2,4-DICHLORO-6-(3,4,5-TRICHLORO-1H-PYRROL-2YL)PHENOL | C10 H4 Cl5 N O | 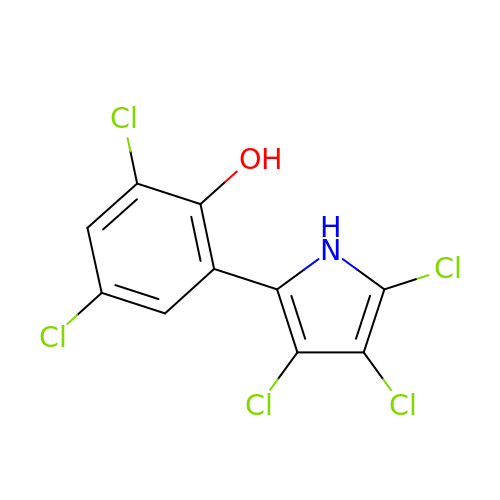FBRLLYYPGGXCKT-UHFFFAOYSA-N> GAMESLPVIAAPSMWTRPQIKDFKEKIQQDADSVITVGRGEVVTVRVPTHEEGSYLFWEFATDNYDIGFGVYFEWTDSPNTAVSVHVSESSDDDEEEEENIGCEEKAKKNANKPLLDEIVPVYRRDCHEEVYAGSHQYPGRGVYLLKFDNSYSL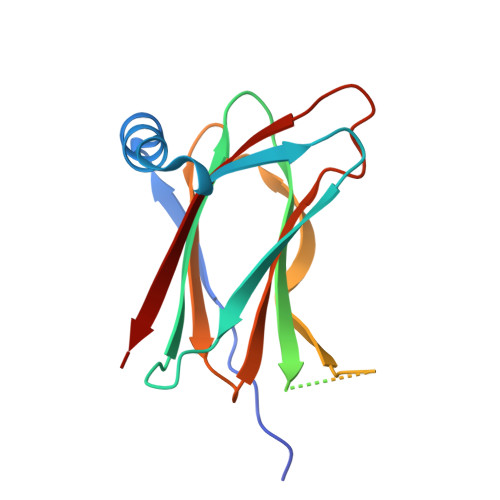WRSKSVYYRVYYTR>[4x]MRAVVFENKERVAVKEVNAPRLQHPLDALVRVHLAGICGSDLHLYHGKIPVLPGSVLGHEFVGQVEA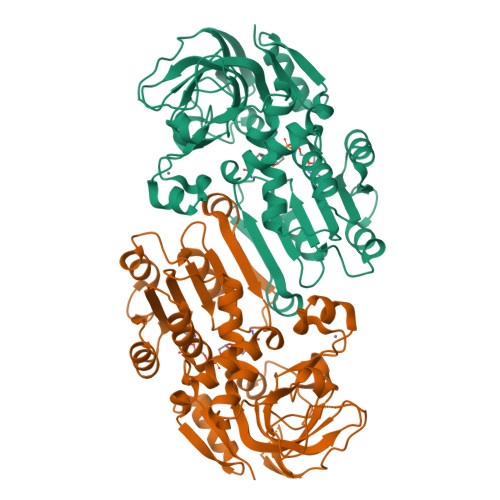VGEGIQDLQPGDWVVGPFHIACGTCPYCRRHQYNLCERGGVYGYGPMFGNLQGAQAEILRVPFSNVNLRKLPPNLSPERAIFAGDILSTAYGGLIQGQLRPGDSVAVIGAGPVGLMAIEVAQVLGASKILAIDRIPERLERAASLGAIPINAEQENPVRRVRSETNDEGPDLVLEAVGGAATLSLALEMVRPGGRVSAVGVDNAPSFPFPLASGLVKDLTFRIGLANVHLYIDAVLALLASGRLQPERIVSHYLPLEEAPRGYELFDRKEALKVLLVVRG Voltage-gated sodium channels are transmembrane proteins responsible for the generation of action potentials in excitable cells and play important roles in the propagation of electrical impulses throughout nerves. They are complexes of a pore-forming α subunit and auxiliary β subunits, designated β1/β1B–β4 (encoded by SCN1B–4B). In addition to the channel modulation, the β subunits function as cell adhesion molecules. In this study, we determined the crystal structures of the mouse and human β4ex proteins containing all three Cys residues, which revealed the formation of a dimer in a parallel arrangement, mediated by the intermolecular disulfide bond and the exchange of the N-terminal segments.

In this study, the human β4ex containing all of the Cys residues was prepared, and its crystal structure was determined in the hexagonal form at 2.2-Å resolution. The human β4ex also assumes the same parallel arrangement as those in the previous and present mouse β4ex crystals. Therefore, it appears that the parallel arrangement of β4 is a conserved natural property. The anti-parallel arrangement was not observed in the cubic and hexagonal crystal forms, probably because PEG fragments were bound to the trans homophilic interface (hexagonal form) and because detergent was used for the crystallization and the C-terminal tag sequence was present (cubic form) (see “Experimental Procedures”). The parallel arrangement of the β4 molecules was mediated, in common, through two types of interactions. First, the β4ex structure forms the intermolecular disulfide bond (the S–S interaction) between the “unpaired” Cys residue (Cys58) in the loop connecting strands B and C. Second, the N-terminal segment Ser30-Val35, which is deleted in another structure of β4ex, is involved in an intermolecular interaction between the two β4ex molecules in the parallel arrangement. This type of interaction is designated hereafter as the N–N interaction. Moreover, in this N–N interaction, the N-terminal segments form hydrogen bonds between their Glu32 and Ser34 with Ser56 and Thr54, respectively, and join the β sheets of the counterparts. As these intermolecular interactions are sophisticated and conserved in the human and mouse β4 structures, we hereafter designate the two β4ex molecules in the parallel arrangement as the parallel dimer.

>SLEVSVGKATDIYAVNGTEILLPCTFSSCFGFEDLHFRWTYNSSDAFKILIEGTVKNEKSDPKVTLKDDDRITLVGSTKEKMNNISIVLRDLEFSDTGKYTCHVKNPKENNLQHHATIFLQVV[2x]> GSHMEEKEILWNEAKAFIAACYQELGKAAEVKDRLADIKSEIDLTG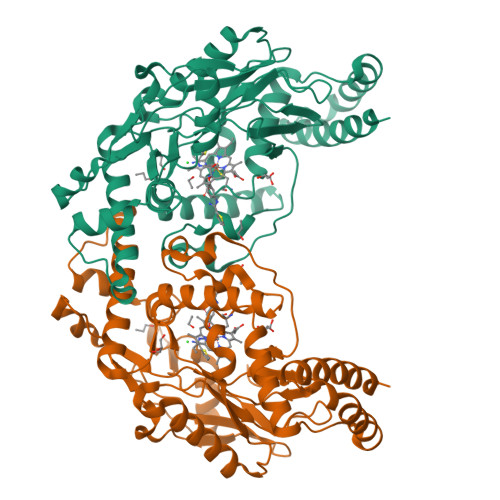SYVHTKEELEHGAKMAWRNSNRCIGRLFWNSLNVIDRRDVRTKEEVRDALFHHIETATNNGKIRPTITIFPPEEKGEKQVEIWNSQLIRYAGYESDGERIGDPASCSLTAACEELGWRGERTDFDLLPLIFRMKGDEQPVWYELPRSLVIEVPITHPDIEAFSDLELKWYGVPIISDMKLEVGGIHYNAAPFNGWYMGTEIGARNLADEKRYDKLKKVASVIGIAADYNTDLWKDQALVELNKAVLHSYKKQGVSIVDHHTAASQFKRFEEQAEEAGRKLTGDWTWLIPPISPAATHIFHRSYDNSIVKPNYFYQDKPYE> MRLLVTGGAGFIGSHFVRQLLAGAYPDVPADEVIVLDSLTYAGNRANLAPVDADPRLRFVHGDIRDAGLLARELRGVDAIVHFAAESHVDRSIAGASVFTETNVQGTQTLLQCAVDAGVGRVVHVSTNQVYGSIDSGSWTESSPLEPNSPYAASKAGSDLVARAYHRTYGLDVRITRCCNNYGPYQHPEKLIPLFVTNLLDGGTLPLYGDGANVREWVHTDDHCRGIALV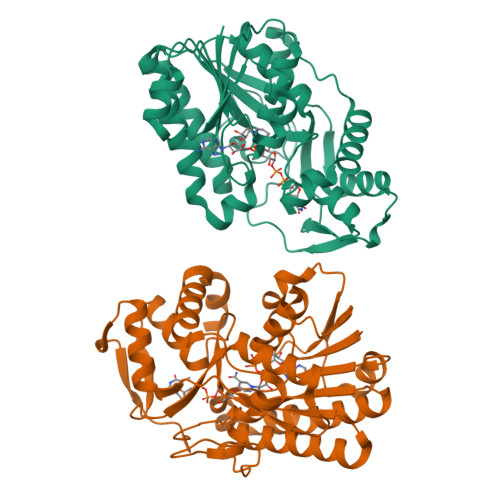LAGGRAGEIYHIGGGLELTNRELTGILLDSLGADWSSVRKVADRKGHDLRYSLDGGKIERELGYRPQVSFADGLARTVRWYRENRGWWEPLKATAPQLPATAVEVSA> HHHHHHMHTSTTSTVPLEPWTAQQLQQATQGYWHKDQIPQTEIKRILTDSRHAESGDAFLALKGERFDAHNFVAQVVANGCQVAIVERPIDAEIAQLVVADTRLALGQLGAYRREQNAQLKVIALTGSSGKTTTKEMLGSILSRLAPTLITRGNLNNDLGVPMMLLELRKEHQYAVMELGANHQGEIDYTSKIVQPHVAGILNIGTAHLGEFGGRDGICRAKSEIYRHILPQGVAIVPQQDDFTAEIREAAKSHQIMSFGEGGDVFATEIELLPQSANFQLHTPQGSSFVRLPFAGEHNVQNATAAVAFALALGVSLEDIVKGLEQAQGAKGRLNFIQKAPHLFIDDTYNANPTSMRAAAQVLLQQNGIKVMVMGDIGELGDSSWQEHHDLGRDLAELPLDHIVAVGQFASAALEGAGLHSTKLKAFQTQAE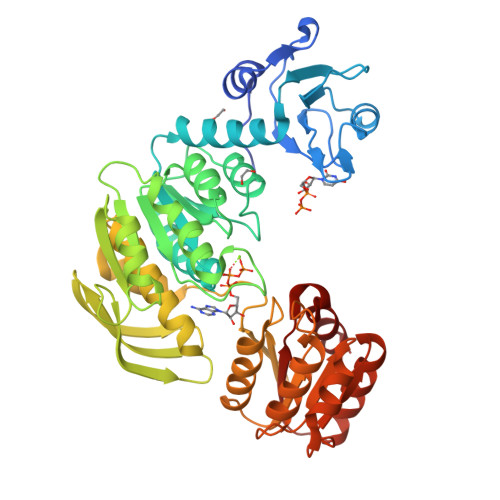ALPFLINLIQTHQPQSMSFLFKGSRFTHMETLMADLMEKL>[2x]HSQITLRGNAINTVGELPAVGSPAPAFTL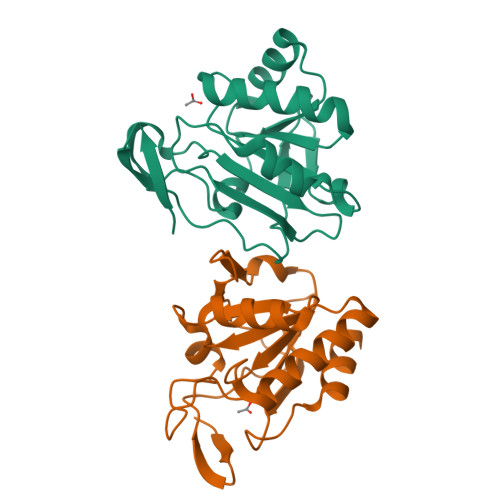TGGDLGVISSDQFRGKSVLLNIFPSVDTPVSATSVRTFDERAAASGATVLCVSKDLPFAQKRFCGAEGTENVMPASAFRDSFGEDYGVTIADGPMAGLLARAIVVIGADGNVAYTELVPEIAQEPNYEAALAALGA>NLPTAQEVQGLMARYIELVDVGDIEAIVQMYADDAT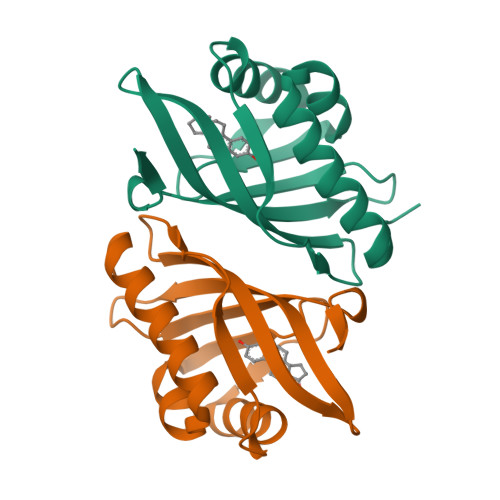VEDPFGQPPIHGREQIAAFYRQGLGGGKVRACLTGPVRASHNGCGAMPFRVEMVWNGQPCALDVIDVMRFDEHGRIQTKQAYWSEVNLSVR[2x]>[2x]MADPRTDNRNRKIPDAQVDAIKVPPHSLEAEQSVIGGLLLDNERWDTVSEHVMTQDFYSRPHRLIFDGVKSILEAGKPLDLITLSEYLEQREQLEDVGGFAYLADLAKNTPSAANINAYAEIVAERALVRNLIGVANEIADAGYDPQGRNAEDLLDLAESKVFAIAEARTSENEGPKNVDSILERTLERIELLYKTPQDGVTGVNTGFTDLNKKTAGLQGSDLIIVAARPSMGKTTFAMNLCENAAMEQDKPVLIFSLEMPAEQIMMRMLAS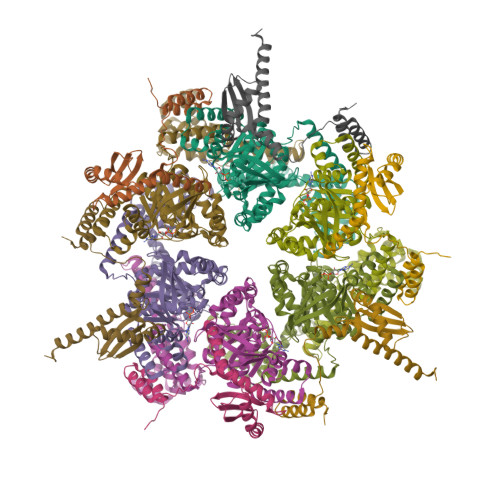LSRVDQTKIRTGQLDDEDWARISSTMGILMEKKNMYIDDSSGLTPTEVRSRARRIAREHGGLSLIMVDYLQLMRVPALTDNRTLEIAEISRSLKALAKELNVPVVALSQLNRSLEQRADKRPVNSDLRESGSIEQDADLIMFIYRDEVYHPDSPLKGTAEIIIGKQRNGPIGSVRLTFQGHYSRFDNYAGPAFDDEHHHHHH;>[2x]MHHHHHHRDHRPTATDELIQASKLKQIQEHAKAILLINRQLQDILPKGLKTQVRAANVRGGNLVLEAASAALKMKVDYERLHILTQLRQNGFGHLISIEVRVNPELYRQSKITSEDARAANPRPPLSEHAAHVLLAIADQASDKVKKRLQSLARLAKANQKDD> MNGVYDVGGTDGLGPINRPADEPVFRAEWEKVAFAMFPATFRAGFMGLDEFKFGIEQMNPAEYLESPYYWHWIRTYIHHGVRTGKIDLEELERRTQYYRENPDAPLPEHEQKPELIEFVNQAVYGGLPASREVDRPPKFKEGDVVRFSTASP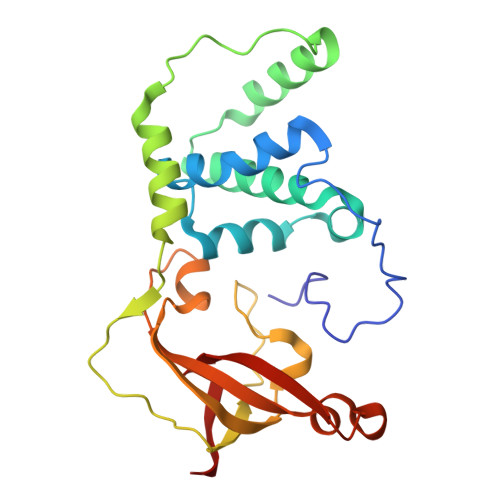KGHARRARYVRGKTGTVVKHHGAYIYPDTAGNGLGECPEHLYTVRFTAQELWGPEGDPNSSVYYDCWEPYIELVDT> SNVRATYTVIFKNASGLPNGYDNWGWGCTLSYYGGAMIINP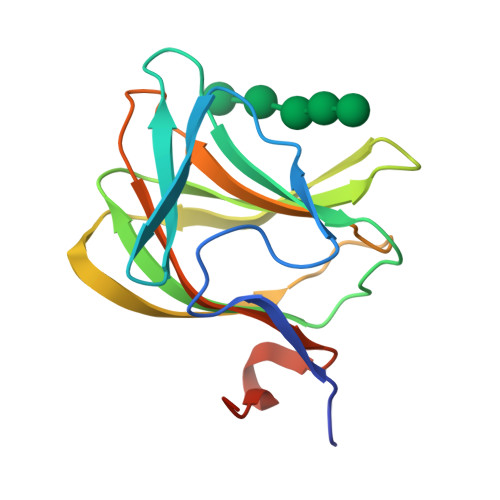QEGKYGAVSLKRNSGSFRGGSLRFDMKNEGKVKILVENSEAAEKFEVETISPSDEYVTYILDVDFDLPFDRIDFQDAPGNGDRIWIKNLVHSTGSADDFVDPINLEHH>[2x]MLITDTLSPQAFEEALRAKGDFYHIHHPYHIAMHNGNATREQIQGWVANRFYYQTTIPLKDAAIMANCPDAQTRRKWVQRILDHDGSHGEDGGIEAWLRLGEAVGLSRDDLLSERHVLPGVRFAVDAYLNFARRACWQEAACSSLTELFAPQISQSRLDSWPQHYPWIKEEGYFYFRSRLSQANRDVEHGL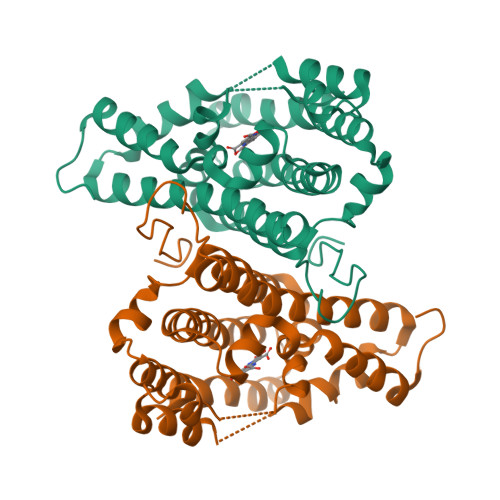ALAKAYCDSAEKQNRMLEILQFKLDILWSMLDAMTMAYALQRPPYHTVTDKAAWHTTRLVLEHHHHH>SNAMNDIVASTQLPNTIKTITNDLRKLGLKKGMTVIVHSSLSSIGWISGGAVAVVEALMEVITEEGTIIMPTQSSDLSDPKHWSRPPVPEEWWQIIRDNVPAFEPHITPTRAMGKVVECFRTYPNV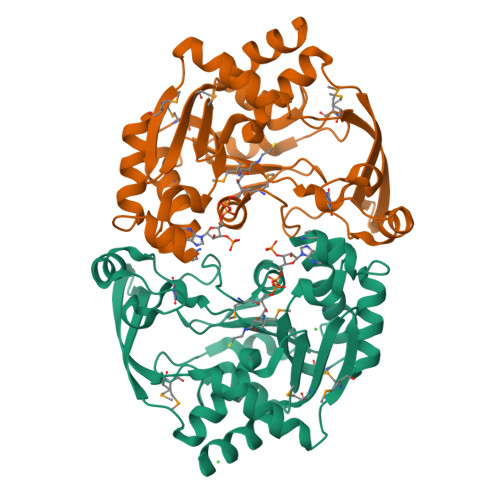VRSNHPLGSFAAWGRHAEEITVNQSLSMSLGEESPLRKIYDLDGYILLIGVGYDSNTSVHLSEVRSGACELIKVGAPIIENGERVWKEFVDMDYDSDKFVEIGVEFEQKGTVTMGKIGNAKCRLMKQRDIVDFGTEWFRKKN[2x]methyl 3-O-((7-carboxy) quinolin-2-yl)-methyl)-beta-D-galactopyranoside 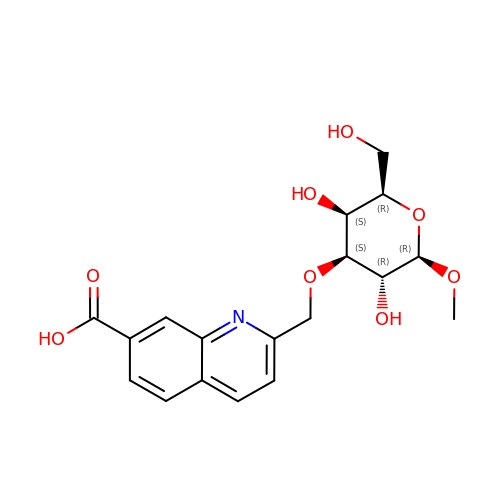| C18 H21 N O8 | OBYVIVUJQDGTKI-RIUYPTKQSA-N> MAPQIRSRSLAAQEPASVLEEARLRLHVSAVPESLPCREQEFQDIYNFVESKLLDHTGGCMYISGVPGTGKTATVHEVIRCLQQAAQANDVPPFQYIEVNGMKLTEPHQVYVQILQKLTGQKATANHAAELLAKQFCTRGSPQETTVLLVDELDLLWTHKQDIMYNLFDWPTHKEARLVVLAIANTMDLPERIMMNRVSSRLGLTRMCFQPYTYSQLQQILRSRLKHLKAFEDDAIQLVARKVAALSGDARRCLDICRRATEICEFSQQKPDSPGLVTIAHSMEAVDEMFSSSYITAIKNSSVLEQSFLRAILAEFRRSGLEEATFQQIYSQHVALCRMEGLPYPTMSETMAVCSHLGSCRLLLVEPSRNDLLLRVRLNVSQDDVLYALKDE;> MSKPELKEDKMLEVHFVGDDDVLNHILDREGGAKLKKERAQLLVNPKKIIKKPEYDLEEDDQEVLKDQNYVEIMGRDVQESLKNGSATGGGNKVYSFQNRKHSEKMAKLASELAKTPQKSVSFSLKNDPEITINVPQSSKGHSASDKVQPKNNDKSEFLSTAPRSLRKRLIVPRSHSDSESEYSASNSEDDEGVAQEHEEDTNAVIFSQKIQAQNRVVSAPVGKETPSKRMKRDKTSDLVEEYFEAHSSSKVLTSDRTLQKLKRAKLDQQTLRNLLSKVSPSFSAELKQLNQQYEKLFHKWMLQLHLGFNIVLYGLGSKRDLLERFRTTMLQDSIHVVINGFFPGISVKSVLNSITEEVLDHMGTFRSILDQLDWIVNKFKEDSSLELFLLIHNLDSQMLRGEKSQQIIGQLSSLHNIYLIASIDHLNAPLMWDHAKQSLFNWLWYETTTYSPYTEETSYENSLLVKQSGSLPLSSLTHVLRSLTPNARGIFRLLIKYQLDNQDNPSYIGLSFQDFYQQCREAFLVNSDLTLRAQLTEFRDHKLIRTKKGTDGVEYLLIPVDNGTLTDFLEKEEEEA;> MATSSMSKGCFVFKPNSKKRKISLPIEDYFNKGKNEPEDSKLRFETYQLIWQQMKSENERLQEELNKNLFDNLIEFLQKSHSGFQKNSRDLGGQIKLREIPTAALVLGVNVTDHDLTFGSLTEALQNNVTPYVVSLQAKDCPDMKHFLQKLISQLMDCCVDIKSKEEESVHVTQRKTHYSMDSLSSWYMTVTQKTDPKMLSKKRTTSSQWQSPPVVVILKDMESFATKVLQDFIIISSQHLHEFPLILIFGIATSPIIIHRLLPHAVSSLLCIELFQSLSCKEHLTTVLDKLLLTTQFPFKINEKVLQVLTNIFLYHDFSVQNFIKGLQLSLLEHFYSQPLSVLCCNLPEAKRRINFLSNNQCENIRRLPSFRRYVEKQASEKQVALLTNERYLKEETQLLLENLHVYHMNYFLVLRCLHKFTSSLPKYPLGRQIRELYCTCLEKNIWDSEEYASVLQLLRMLAKDELMTILEKCFKVFKSYCENHLGSTAKRIEEFLAQFQSLDAETKEEEDASGSQPKGLQKTDLYHLQKSLLEMKELRRSKKQTKFEVLRENVVNFIDCLVREYLLPPETQPLHEVVYFSAAHALREHLNAAPRIALHTALNNPYYYLKNEALKSEEGCIPNIAPDICIAYKLHLECSRLINLVDWSEAFATVVTAAEKMDANSATSEEMNEIIHARFIRAVSELELLGFIKPTKQKTDHVARLTWGGC;> MSSRKSKSNSLIHTECLSQVQRILRERFCRQSPHSNLFGVQVQYKHLSELLKRTALHGESNSVLIIGPRGSGKTMLINHALKELMEIEEVSENVLQVHLNGLLQINDKIALKEITRQLNLENVVGDKVFGSFAENLSFLLEALKKGDRTSSCPVIFILDEFDLFAHHKNQTLLYNLFDISQSAQTPIAVIGLTCRLDILELLEKRVKSRFSHRQIHLMNSFGFPQYVKIFKEQLSLPAEFPDKVFAEKWNENVQYLSEDRSVQEVLQKHFNISKNLRSLHMLLMLALNRVTASHPFMTAVDLMEASQLCSMDSKANIVHGLSVLEICLIIAMKHLNDIYEEEPFNFQMVYNEFQKFVQRKAHSVYNFEKPVVMKAFEHLQQLELIKPMERTSGNSQREYQLMKLLLDNTQIMNALQKYPNCPTDVRQWATSSLSWL;> MPHLENVVLCRESQVSILQSLFGERHHFSFPSIFIYGHTASGKTYVTQTLLKTLELPHVFVNCVECFTLRLLLEQILNKLNHLSSSEDGCSTEITCETFNDFVRLFKQVTTAENLKDQTVYIVLDKAEYLRDMEANLLPGFLRLQELADRNVTVLFLSEIVWEKFRPNTGCFEPFVLYFPDYSIGNLQKILSHDHPPEYSADFYAAYINILLGVFYTVCRDLKELRHLAVLNFPKYCEPVVKGEASERDTRKLWRNIEPHLKKAMQTVYLREISSSQWEKLQKDDTDPGQLKGLSAHTHVELPYYSKFILIAAYLASYNPARTDKRFFLKHHGKIKKTNFLKKHEKTSNSLLGPKPFPLDRLLAILYSIVDSRVAPTANIFSQITSLVTLQLLTLVGHDDQLDGPKYKCTVSLDFIRAIARTVNFDIIKYLYDFL

The very first step of this initiation process is accomplished by DNA association with the Origin Recognition Complex (ORC), a six-subunit protein that forms a partial ring around origin DNA. The complex consists of six subunits (ORC1-6), with subunits ORC1-5 forming a partial ring capable of encircling DNA. All five subunits contain a winged-helix domain (WHD) and a AAA+ domain which consists of the RecA-fold and lid domains, although the ORC2 and ORC3 RecA-folds have diverged slightly and do not contain a lid domain. Adjacent ORC subunits associate in a double-layer arrangement through interfaces between the WHDs in one layer and the AAA+ domains in another with ATP-binding sites sandwiched between the ORC1·4, ORC4·5, and ORC5·3 AAA+ interfaces (Tocilj et al., 2017).

In contrast to ORCO2WH, ORCO1AAA consists of a dynamic ORC2 WHD that is unresolved in the refined map. The ORC1 AAA+ domain in this structure is ordered and forms the important interface with ORC4 with an ATP coordinated between the two subunits, an ATPase active conformation seen in previous ScORC and HsORC structures. In the ORCO1AAA structure, the ORC2 WHD undergoes conformational changes but does not change its overall position in the complex. While ORC1 AAA+ is locked in the auto-inhibited state in DmORC, the ORC1 AAA+ domain in human ORC appears to be dynamic along a continuum of positions between two extreme states: the auto-inhibited state observed in the DmORC and when it forms the ORC1·4 interface with ORC4 as observed in ORCO1AAA. ORCO1AAA was especially improved in this region due to the 3D focused refinement we applied. The homologous ORC4 region in HsORC is visible in the ORCO1AAA cryoEM density map allowing us to now model this region. This region in HsORC is 20 residues shorter than the ScORC segment and does not contain an α-helix (Hu et al., 2020). The missing helix in HsORC likely reduces its ability to bind specifically to a DNA sequence resulting in the requirement of other mechanisms to establish stable origin interactions. Overall, the ORCO1AAA and ORCO2WH populations reveal a dynamic switch between the ORC1 AAA+ and ORC2 WHD where the locking into position of one domain within the ORC ring-shaped core kicks the other domain into a dynamic state.(E)-N-({3-hydroxy-2-methyl-5-[(phosphonooxy)methyl]pyridin-4-yl}methylidene)-3-[(3S)-2-oxo-2,3-dihydro-1H-indol-3-yl]-L-alanine 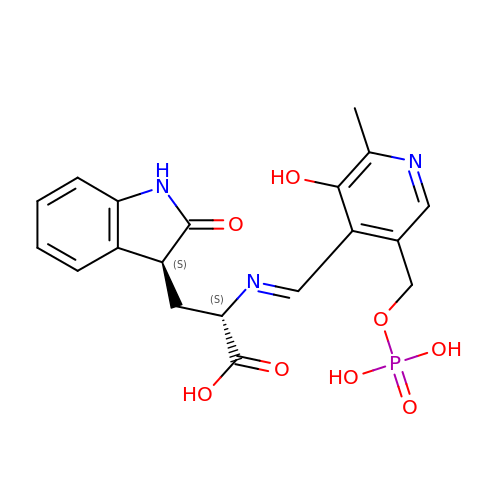| C19 H20 N3 O8 P | ZXXYWPJNDHLAKD-ARQPKOPCSA-N Here, we characterize the structure and function of a thermophilic dNDT, the protein from Chroococcidiopsis thermalis (CtNDT). Nucleoside 2′-deoxyribosyltransferase (dNDT) enzymes catalyze transglycosylation via a covalent 2′-deoxyribosylated enzyme intermediate with retention of configuration, having applications in the biocatalytic synthesis of 2′-deoxynucleoside analogues in a single step. The reaction catalyzed by dNDT proceeds via a ping-pong mechanism, with the formation of a 2′-deoxyribosyl-enzyme intermediate covalently linked to an active-site glutamate.13 Transglycosylation occurs in a stereospecific manner, preserving the anomeric carbon in the β configuration in the newly formed 2′-deoxyribonucleoside. As with other NDT enzymes, the active site of CtNDT is formed by residues from two monomers, and therefore, it is only fully formed in the dimer/tetramer.

We compared two potential transition-state analogues for transglycosylation, immucillin-H (ImmH) and DADme–immucillin-H (DADmeH), as the distance between the bond being broken/formed in the nucleobase and sugar varies. Enzymes evolved to bind tightly to their cognate transition state and therefore to stable compounds that most closely mimic the charge distribution and geometry of that transition state. Based on Scheme 1 and considering 2′-deoxyribonucleside1 as a substrate, releasing nucleobase1 and generating a 2′-deoxyribosylated enzyme, ImmH would mimic an early transition state in which the distance between ribose C1′ and the nucleobase is ∼1.5 Å, while DADmeH would mimic a late transition state, since the presence of a methylene bridge between ribitol N1′ (which replaces C1′ in DADmeH) keeps the nucleobase at a distance of ∼3.0 Å from these groups. Structures were obtained with the two potential transition-state analogues ImmH and DADmeH. The structure of bound ImmH largely resembles that of the clofarabine-bound complex, in agreement with the relatively weak binding of ImmH to CtNDT, and it is therefore substrate-like. For ImmH, ΔH was −5.25 ± 0.07 kcal mol–1, −TΔS was −0.36 ± 0.14 kcal mol–1, and KD was 78.2 ± 6.6 μM, while for DADmeH, ΔH was −11.43 ± 0.29 kcal mol–1, −TΔS was 0.38 ± 0.73 kcal mol–1, and KD was 9 ± 5 nM. ΔG was −5.60 ± 0.08 for ImmH and −11.05 ± 0.42 kcal mol–1 for DADmeH; therefore, binding is determined by an enthalpic contribution. Although no signal change was observed with DADmeH, ImmH binding led to a small fluorescence decrease in a single transient. Computational studies proposed the formation of an oxocarbenium ion in the transition state for the reaction, and D62 is equivalent to a residue proposed to interact with the anomeric carbon in this putative oxocarbenium ion transition state. CtNDTD62N, however, retained ∼50% catalytic efficiency in comparison to WT, and it is unlikely to play such a crucial role in transition-state stabilization.

>[2x]MKRKIIYLASPYGFSQQQKTLLLPPIVRALEALGIEVWEPFARNNQIDFSQADWAYRVAQANLQDVKNCDGIFAVVNGTPPDEGVMVELGMAIALNKAIFLFRDDFRRCSDNERYPLNLMLFAGLPEIGWENYYYTSVDEIQSHDKALYKWLTGM Hexon is a trimeric, barrel-shaped protein that represents the main building block of the virus capsid. Adenoviruses are non-enveloped viruses with a capsid of icosahedral symmetry that encapsulates a double-stranded DNA genome. In this model, human lactoferrin (hLF), an innate immune protein, aids the viral uptake into epithelial cells by mediating interactions between the major capsid protein, hexon, and yet unknown host cellular receptor(s). Here, we present a new cryo-EM structure of HAdV-5C hexon at high resolution alongside a hybrid structure of HAdV-5C hexon complexed with human lactoferrin (hLF).

The structure of the HAdV-C5 hexon was reconstructed to FSC0.143 of 2.9 Å. To our knowledge, this is the highest resolution structure of HAdV-C5 hexon determined by cryo-EM. Due to the high stability of the trimer, the resolution is relatively uniform across the whole structure and thus it could be modeled unambiguously with a high average cross-correlation of 0.736. Throughout the length of the hexon, the protomers are in close contact forming large interfaces in addition to intertwined regions at the “turrets” and the base. Each protomer contributes approximately 16,000 Å2 to the interface with the two other protomers. Significantly lower resolution is observed only for the hypervariable loop regions, the “turrets” at the top of the molecule which are largely disordered and could not be built due to a lack of traceable density in the final reconstruction. Specifically, regions 137–164, 188–190, 252–256, 271–278, and 431–436 could not be sufficiently reconstructed. The same structure was used as a starting model to build hexon in the cryo-EM reconstruction but no major conformational changes were observed. The RMSD between both structures is 0.9 Å, indicating high overall similarity.

>[3x]MATPSMMPQWSYMHISGQDASEYLSPGLVQFARATETYFSLNNKFRNPTVAPTHDVTTDRSQRLTLRFIPVDREDTAYSYKARFTLAVGDNRVLDMASTYFDIRGVLDRGPTFKPYSGTAYNALAPKGAPNPCEWDEAATALEINLEEEDDDNEDEVDEQAEQQKTHVFGQAPYSGINITKEGIQIGVEGQTPKYADKTFQPEPQIGESQWYETEINHAAGRVLKKTTPMKPCYGSYAKPTNENGGQGILVKQQNGKLESQVEMQFFSTTEATAGNGDNLTPKVVLYSEDVDIETPDTHISYMPTIKEGNSRELMGQQSMPNRPNYIAFRDNFIGLMYYNSTGNMGVLAGQASQLNAVVDLQDRNTELSYQLLLDSIGDRTRYFSMWNQAVDSYDPDVRIIENHGTEDELPNYCFPLGGVINTETLTKVKPKTGQENGWEKDATEFSDKNEIRVGNNFAMEINLNANLWRNFLYSNIALYLPDKLKYSPSNVKISDNPNTYDYMNKRVVAPGLVDCYINLGARWSLDYMDNVNPFNHHRNAGLRYRSMLLGNGRYVPFHIQVPQKFFAIKNLLLLPGSYTYEWNFRKDVNMVLQSSLGNDLRVDGASIKFDSICLYATFFPMAHNTASTLEAMLRNDTNDQSFNDYLSAANMLYPIPANATNVPISIPSRNWAAFRGWAFTRLKTKETPSLGSGYDPYYTYSGSIPYLDGTFYLNHTFKKVAITFDSSVSWPGNDRLLTPNEFEIKRSVDGEGYNVAQCNMTKDWFLVQMLANYNIGYQGFYIPESYKDRMYSFFRNFQPMSRQVVDDTKYKDYQQVGILHQHNNSGFVGYLAPTMREGQAYPANFPYPLIGKTAVDSITQKKFLCDRTLWRIPFSSNFMSMGALTDLGQNLLYANSAHALDMTFEVDPMDEPTLLYVLFEVFDVVRVHRPHRGVIETVYLRTPFSAGNATT Tetrahydrodeoxycorticosterone | C21 H34 O3 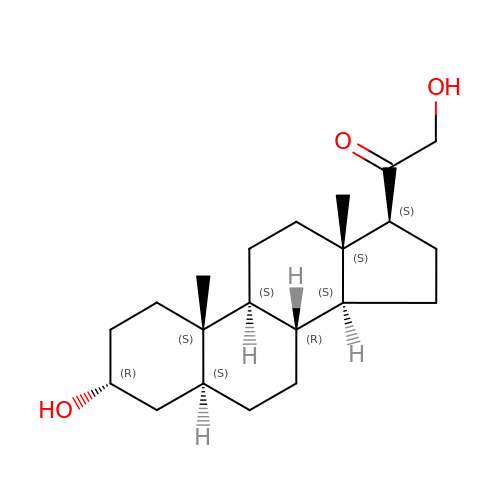| CYKYBWRSLLXBOW-GDYGHMJCSA-N> ACTTCCAGTCCGTGGTAGGGCAGGTTGGGGTGACCGCTATAT;> ATATAGCGTGG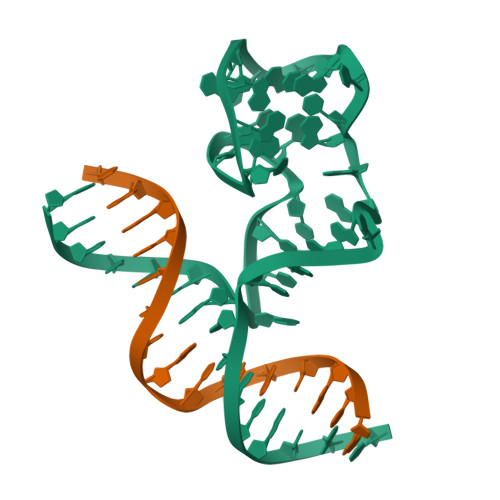AAGT> GHMSVYHHILLAVDFSSEDSQVVQKVRNLASQIGARLSLIHVLDNIPMPDTPYGTAIPLDTETTYDAMLDVEKQKL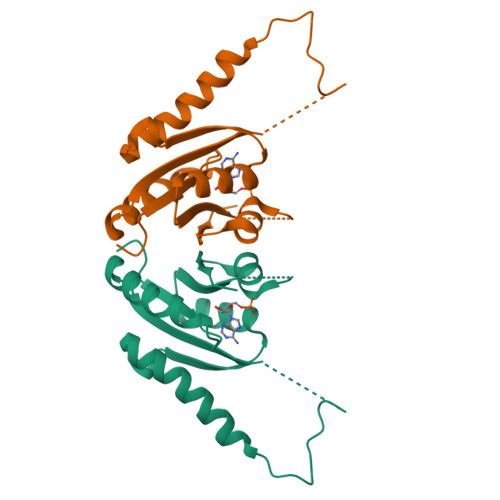SQIGNTLGIDPAHRWLVWGEPREEIIRIAEQENVDLIVVGSHGRHGLALLLGSTANSVLHYAKCDVLAVRLRDD>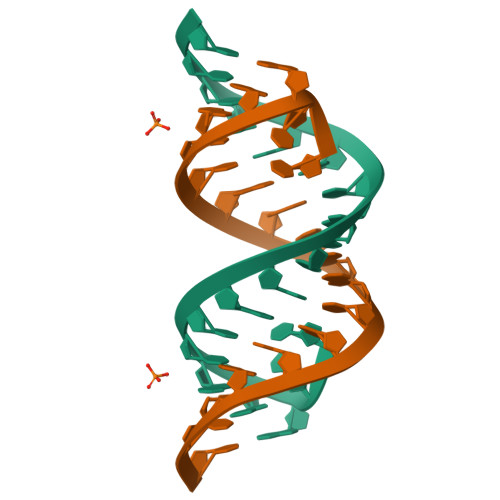UUGGGCCAGCAGCAGGUCC[2x]> GAGCAGACG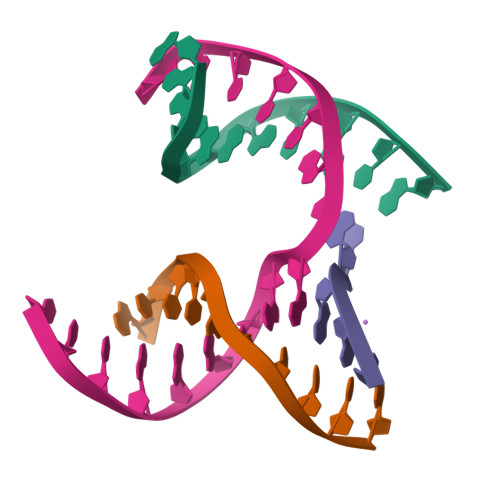TGGAGCAGACGTG;> ACCCCACTCA;> CAGGT;> TCTGAGTGGCGTCTGC>[4x]MSLAWLISEFASVGD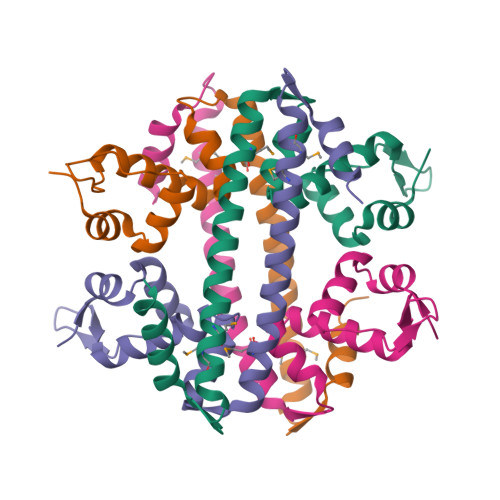VTVRALRYYDKINLLKPSDYTEGGHRLYTKDDLYVLQQIQSFKHLGFSLGEIQNIILQRDIETEVFLRQMHFQREVLLAEQERIAKVLSHMDEMTKKFQKEERVNVALFSSFLQTFIWEKENKEGHHHHHH>APKRKAGVSKCETKCTKACPRPAPVPKLLIKGGMEVLDLVTGPDSVTEIEAFLNPRMGQPPTPESLTEGGQYYGWSRGINLATSDTEDSPGNNT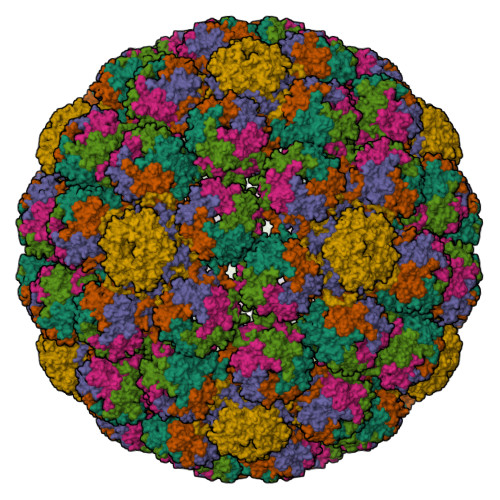LPTWSMAKLQLPMLNEDLTCDTLQMWEAVSVKTEVVGSGSLLDVHGFNKPTDTVNTKGISTPVEGSQYHVFAVGGEPLDLQGLVTDARTKYKEEGVVTIKTITKKDMVNKDQVLNPISKAKLDKDGMYPVEIWHPDPAKNENTRYFGNYTGGTTTPPVLQFTNTLTTVLLDENGVGPLCKGEGLYLSCVDIMGWRVTRNYDVHHWRGLPRYFKITLRKRWVKNPYPMASLISSLFNNMLPQVQGQPMEGENTQVEEVRVYDGTEPVPGDPDMTRYVDRFGKTKTVFPGN[6x]> PKEVYLDRKLLTLEDKELGSGNFGTVKKGYYQMKKVVKTVAVKILKNEANDPALKDELLAEANVMQQLDNPYIVRMIGICEAESWMLVMEMAELGPLNKYLQQNRHVKDKNIIELVHQVSMGMKYLEESNFVHRDLAARNVLLVTQHYAKISDFGLSKALRADENYYKAQTHGKWPVKWYAPECINYYKFSSKSDVWSFGVLMWEAFSYGQKPYRGMKGSEVTAMLEKGERMGCP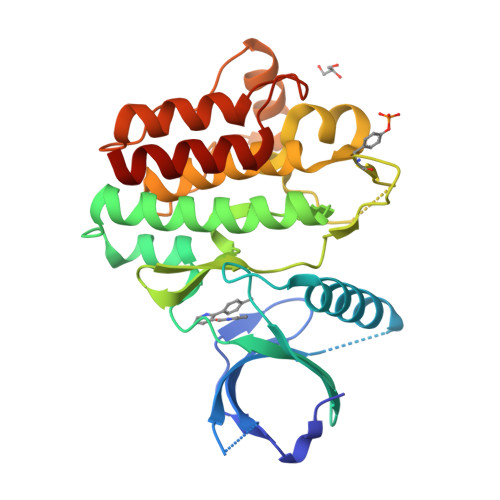AGCPREMYDLMNLCWTYDVENRPGFAAVELRLRNYYYDVVN In metazoans, this post-translational modification is initiated by a large family (20 in humans) of polypeptide N-acetylgalactosaminyltransferases (GalNAc-Ts), which transfer a GalNAc residue from uridine diphosphate N-acetylgalactosamine (UDP-GalNAc) to Ser/Thr side chains in the presence of manganese2. GalNAc-T isoforms contain an N-terminal catalytic domain adopting a GT-A fold and a unique C-terminal lectin domain, classified as a carbohydrate-binding module (CBM) 13 in the CAZy database, with a β-trefoil fold that are connected through a short flexible linker. A key structural feature of these enzymes in catalysis is the existence of a flexible loop formed by residues Arg362 to Ser373 (residue numbers in GalNcAc-T2) that adopts different conformations during the catalytic cycle and renders the enzyme catalytically inactive or active. Here we present the first crystal structures of the inactivated and activated forms of the GalNAc-T2 isoform in binary and ternary complexes with different GalNAc-glycopeptides enabling us to study in detail the lectin-mediated modulatory mechanism of catalysis.

Despite the co-crystallization experiments were performed with GalNAc-T2, UDP and Mn+2, we obtained binary complexes with glycopeptides MUC5AC-Cys13 and MUC5AC-3-13 (the binary complexes are referred to the enzyme complexed to the different glycopeptides MUC5AC-Cys13 and MUC5AC-3-13, respectively), and a ternary complex with MUC5AC-13 (the ternary complex is referred to the enzyme bound to UDP and the glycopeptide MUC5AC-13). Interestingly, MUC5AC-13 was bound to an active form of GalNAc-T2, whereas MUC5AC-Cys13 and MUC5AC-3-13 were unpredictably trapped bound to the inactive form of GalNAc-T2. In these cases, the flexible loop was found in an open conformation, different from the one previously described for the GalNAc-T2-UDP complex (PDB entry 2FFV14 and root-mean-square deviation (RMSD) of 4.68 Å for aligned Cα atoms corresponding to the flexible loop; Fig. 1c,d), which further demonstrates the loop versatility. MUC5AC-13 as well as MUC5AC-Cys13 and MUC5AC-3-13 glycopeptides have a C-terminal GalNAc moiety that establishes interactions with the lectin domain-binding site. The sugar moiety for the three above glycopeptides adopts a perpendicular conformation with respect to the peptide backbone. This also supports previous data suggesting that Cys residues bound to a GalNAc moiety mimic fairly well Thr residues linked to the same sugar. Although the N-terminal of MUC5AC-13 is covered by the flexible loop, the N-termini of MUC5AC-Cys13 and MUC5AC-3-13 are exposed to the solvent and inserted into the sugar nucleotide-binding site. The latter two glycopeptides adopt very similar binding modes, although some differences stand out towards the N-terminus (RMSD of 0.72 Å for aligned Cα atoms corresponding to residues Gly1-Ser5).

> MRRRSRMLLCFAFLWVLGIAYYMYSGGGSALAGGAGGGAGRKEDWNEIDPIKKKDLHHSNGEEKAQSMETLPPGKVRWPDFNQEAYVGGTMVRSGQDPYARNKFNQVESDKLRMDRAIPDTRHDQCQRKQWRVDLPATSVVITFHNEARSALLRTVVSVLKKSPPHLIKEIILVDDYSNDPEDGALLGKIEKVRVLRNDRREGLMRSRVRGADAAQAKVLTFLDSHCECNEHWLEPLLERVAEDRTRVVSPIIDVINMDNFQYVGASADLKGGFDWNLVFKWDYMTPEQRRSRQGNPVAPIKTPMIAGGLFVMDKFYFEELGKYDMMMDVWGGENLEISFRVWQCGGSLEIIPCSRVGHVFRKQHPYTFPGGSGTVFARNTRRAAEVWMDEYKNFYYAAVPSARNVPYGNIQSRLELRKKLSCKPFKWYLENVYPELRVPDHQDIAFGALQQGTNCLDTLGHFADGVVGVYECHNAGGNQEWALTKEKSVKHMDLCLTVVDRAPGSLIKLQGCREDDSRQKWEQIEGNSKLRHVGSNLCLDSRTAKSGGLSVEVCGPALSQQWKFTLNLQQ;> GTTPSPVPTTSTCSAA> 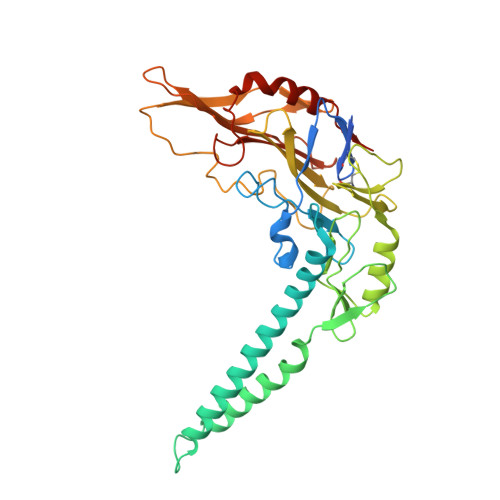MKRVLMGLILLSSSNITWAEAPSSKYQECLGRMTFEIPEEMEWATYDASRVWQISKGGGHNFTAEVTAVGDNGSYDYDSMIFYVSEKVDKNEFHNASNYIKGTAEIYQDHLRENIKLDKKAISTLQKNKSEEKSIERIKKGIAEMEAKIPLAKIYEHDLGIPDSHILGSKNIPFHVLLWRNQRVYYFTFSKPTENSAQRIKDLIARFRTRELYEVPNEPGICFPYGFIADDGKTAYELKNSLRFTRTPNVIFSLLTASANDPWQTRPTSGLYDSDFRPGYDRQKWKKSALLDSLHIGKRLAAFEGWRLDPRPDSGERERAWFGLAHTGGTLDPLVAIQVQTFQKGTDDLTDYTPPPEEVLPRLKALSQSIEQRLAR> MSMEKQVLKENMKTTYHMDGSVDGHYFEIEGEGTGNPFKGEQELKLRVTKGGPLPFAFDILSPTFTYGNRVFTDYPEDMPDYFKQSLPEGYSWERTMMYEDGASATASARISLDKNGF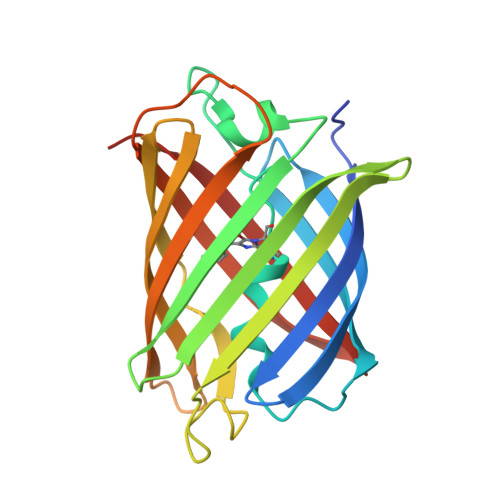VHKSTFHGENFPANGPVMKKKGVDWEPSSETITPEDGILKGDVEMFLVLEGGQRLKALFQTTYKANKVVKMPPRHKIEHRLVRSEDGETIQLQEHAVAKYFTE>MGSSHHHHHHENLYFQGAESTQGQHNYKSLKYYYSKPSIELKNLDGLYRQKVTDKGVYVWKDRKDYFVGLLGKDIEKYPQGEHDKQDAFLVIEEETVNGRQYSI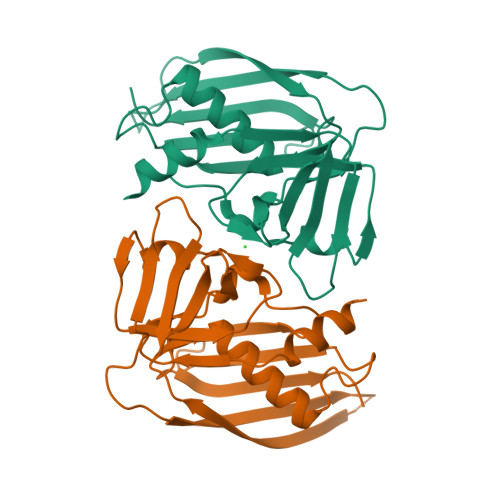GGLSKTNSKEFSKEVDVKVTRKIDESSEKSKDSKFKITKEEISLKELDFKLRKKLMEEEKLYGAVNNRKGKIVVKMEDDKFYTFELTKKLQPHRMGDTIDGTKIKEINVELEYK[4x]>[2x]GRLETQRKKLTVFFSDIRGFTELSEELEAEALTDLLNNYLNEMSKIALKYGGTIDKFVGDCVMVFFGDPSTQGAKKDAVAAVSMGIAMRKHMKVLRQ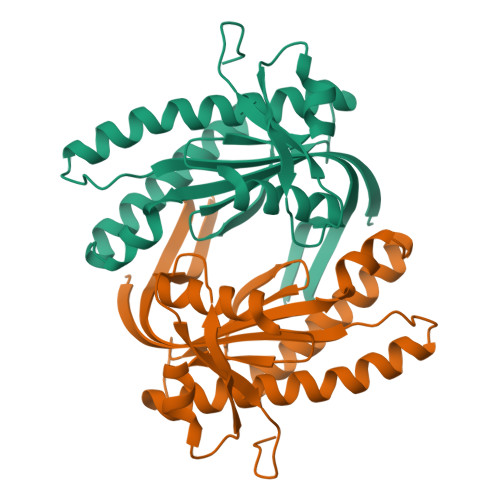QWRAQGITKPLEIRMGINTGYCTVGNFGADTRMDYTIIGREVNLASRLESASEAGEILISHETYSLIKDVIMCRDKGQIAVKGFSRPVQIYQVVDSRRDLG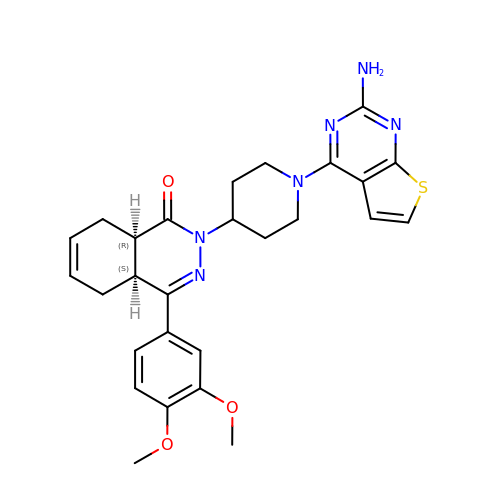(4aS,8aR)-2-(1-{2-aminothieno[2,3-d]pyrimidin-4-yl}piperidin-4-yl)-4-(3,4- dimethoxyphenyl)-1,2,4a,5,8,8a-hexahydrophthalazin-1-one | C27 H30 N6 O3 S | VRSCGUCAJHMOSB-RBUKOAKNSA-N> LVHVASVEKGRSYEDFQKVY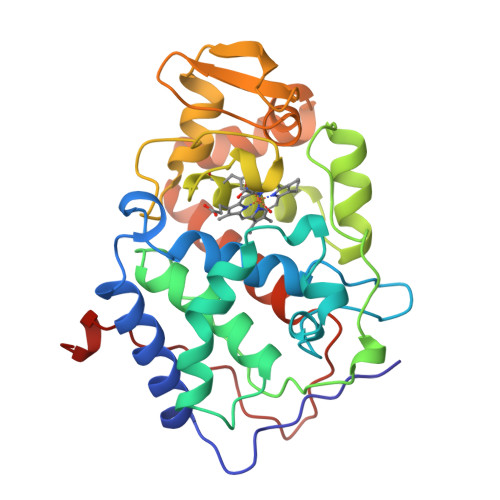NAIALKLREDDEYDNAIGYGPVLVRLAWHISGTWDKHDNTGGSYGGTYRFKKEFNDPSNAGLQNGFKFLEPIHKEFPWISSGDLFSLGGVTAVQEMQGPKIPWRCGRVDTPEDTTPDNGRLPDADKDAGYVRTFFQRLNMNDREVVALMGAHALGKTHLKNSGYEGPWGAANNVFTNEFYLNLLNEDWKLEKNDANNEQWDSKSGYMMLPTDYSLIQDPKYLSIVKEYANDQDKFFKDFSKAFEKLLEDGITFPKDAPSPFIFKTLEEQGL> DDHSELLVNTKSGKVMGTRVPVLSSHISAFLGIPFAEPPVGNMRFRRPEPKKPWSGVWNASTYPNNCQQYVDEQFPGFSGSEMWNPNREMSEDCLYLNIWVPSPRPKSTTVMVWIYGGGFYSGSSTLDVYNGKYLAYTEEVVLVSLSYRVGAFGFLALHGSQEAPGNVGLLDQRMALQ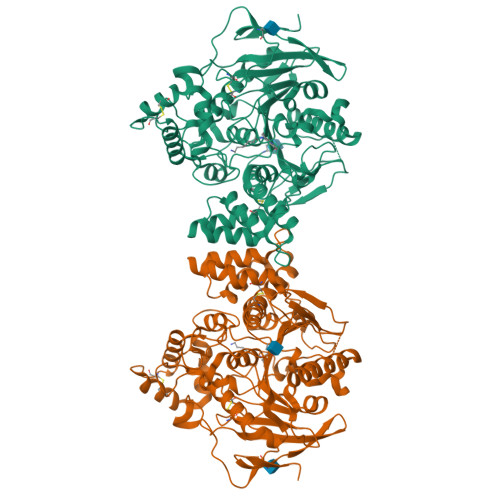WVHDNIQFFGGDPKTVTIFGESAGGASVGMHILSPGSRDLFRRAILQSGSPNCPWASVSVAEGRRRAVELGRNLNCNLNSDEELIHCLREKKPQELIDVEWNVLPFDSIFRFSFVPVIDGEFFPTSLESMLNSGNFKKTQILLGVNKDEGSFFLLYGAPGFSKDSESKISREDFMSGVKLSVPHANDLGLDAVTLQYTDWMDDNNGIKNRDGLDDIVGDHNVICPLMHFVNKYTKFGNGTYLYFFNHRASNLVWPEWMGVIHGYEIEFVFGLPLVKELNYTAEEEALSRRIMHYWATFAKTGNPNEPHSQESKWPLFTTKEQKFIDLNTEPMKVHQRLRVQMCVFWNQFLPKLLNATET{2-[(4-chlorophenyl)methoxy]phenyl}{5-[2-(methylamino)-1,3-thiazol-4-yl]-2,3-dihydro-1H-indol-1-yl}methanone 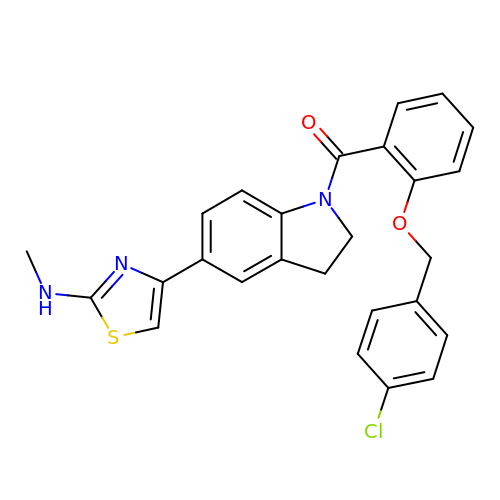| C26 H22 Cl N3 O2 S | GOAZOFMNXDONAU-UHFFFAOYSA-N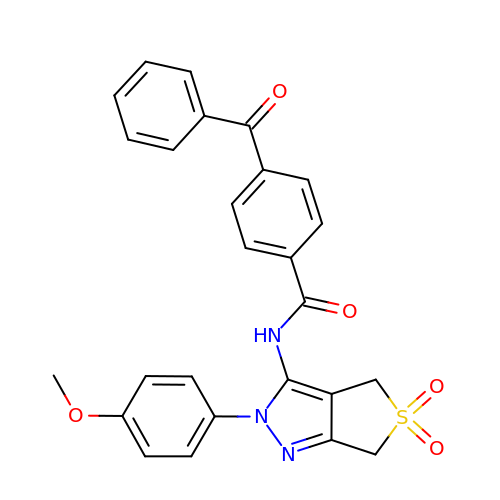N-[2-(4-methoxyphenyl)-5,5-bis(oxidanylidene)-4,6-dihydrothieno[3,4-c]pyrazol-3-yl]-4-(phenylcarbonyl)benzamide | C26 H21 N3 O5 S | FETYBXQBGAFWOV-UHFFFAOYSA-N> GSSRAMGNEVAGVEDISVEITPSSK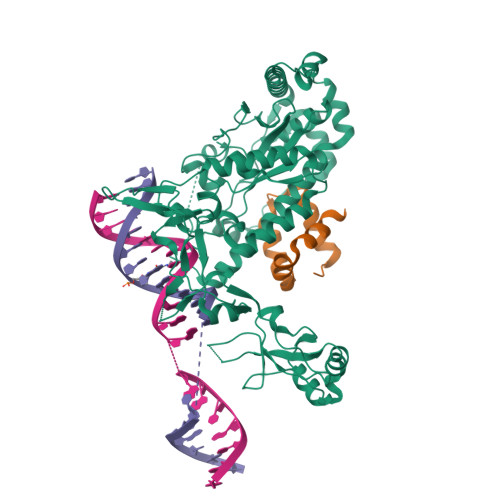RNSDARRTSRNCSSNEERKRRKYFHMLYLVCLMVHGFIRNEWINSKRLSRKLSNLVPEKVFELLHPQKDEELPLRSTRKLLDGLKKCMELWQKHWKITKKYDNEGLYMRTWKEIEMSANNKRKFKTLKRSDFLRAVSKGHGDPDISVQGFVAMLRACNVNARLIMSCQPPDFTNMKIDTSLNGNNAYKDMVKYPIFWCEVWDKFSKKWITVDPVNLKTIEQVRLHSKLAPKGVACCERNMLRYVIAYDRKYGCRDVTRRYAQWMNSKVRKRRITKDDFGEKWFRKVITALHHRKRTKIDDYEDQYFFQRDESEGIPDSVQDLKNHPYYVLEQDIKQTQIVKPGCKECGYLKVHGKVGKVLKVYAKRDIADLKSARQWYMNGRILKTGSRCKKVIKRTVGRPKGEAEEEDERLYSFEDTELYIPPLASASGEITKNTFGNIEVFAPTMIPGNCCLVENPVAIKAARFLGVEFAPAVTSFKFERGSTVKPVLSGIVVAKWLREAIETAIDGIEFI;> GSGNASSGALGTTGGATDAAQGGPPGSIGLTVEDLLSLRQVVSGNPEALAPLLENISARYPQLREHIMANPEVFVSMLLEAVGDNMQDVMEGADDMVEGEDIEVTGEAAAAGLGQGEGEGSFQVDYTPEDDQAISRLCELGFERDLVIQVYFACDKNEEAAANILFSDHAD> GAGTTGGKKDDQALSFLGDTKSASELNPPRLVCPDKPPTLPPREEQVRKAYALPLCELPWDDLGPMLGSGTFGRVYPLRRPACTEVTKGFVGRKFAVKIFWLKRKGMMNLFDTISQGGTPSAEQTDPGTIAAIKSEIRSLPTSSSAFRDMVRIADPTVDVEKIKGMADSLTVETIMKEAKTLRTVINTNGFYTEVGETGTIFTQMEKFVQAHRPEIWSTLSKASQEAQASKYAEIGLADNHWSLPLARVLVKDKNDVKHWALLIELFDGDLQPKTDKTGYSLDGWNAKSGGNVVLREIFSSREALIGLTSKLVKPFVVMQNLYSLGHFAIKPPNLLYKYFPGEKGRASRLSVAAGDFGMAGLLHGDMILRGTLAFMAPEMERVSGGLVAKPSYDVYALALTLASFWTAATELRDHYPWVEKCIKPTLKKMKDAPEFTFLRFASKTGPKLYEADTIYALSTCFAVGGKVEKLYHTGMPLLIRLKLSQMADPEPLARVSMRHARFVFKAYAMLDKLLRAPQSEANAETREEQLKQLQSLHIVQFLLFYLRMEPLTAARDNTQSYRRLARALLDFARLDPVYQAATETVQPLPYEFFTEQKDWQNVKVEVSGSEVDETIRKLRTSLTRDRSLSEDSWADLVDIMFGVSLDGLREVVTRVVYSRKTFLLEEKIGNAVKEAVAATYKFDPNTQLIAEDAPDRLFEVVRTDLGLSYPDDSELGRFLVHRVSKSHTAWATVDRLARQALRLALRREERTRQVYEQLLSGEKPSSESEKAFFDSVFSAVSVVSEANYFGLFWDFPSAGLFGVPPEEMQAYVRKTHLAFVGKMWPVETQKKILEAAVRVTVRGLNASLPASLVDVYATVFAALPTKAPVSPPFLYGLEREEYSSLLFDAKLPEFKEMVAFWATRHELNIAVQTAVGKIPDATNLSDEDIEKQLEGMLPAHLRSPSPARFGWPPEAVADNIRLFIREAKDELALHGPDMVHNRIRVNGRSKPPRRAAFLFHEIFRKAIAFKKDISVLQFNQFFTDILKQSFDPQCRRFIAEVKKRVKSAPAEYVRVADTEAVAPLFEGEGKDILKLVAVDPAARAS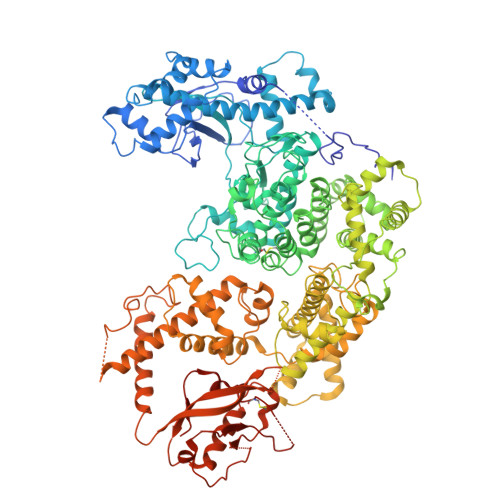DPEPNNCFLWTQAFLDDKTIVVSTGSSGSSGHHHHHHHHHH> MAVASTRLPTVGCSCSVATLAYSRTYVRSSNTRSTGSSSGSIISSSLPWSQHRCQVRTLIVPRQLKAYGGTFSQSIGE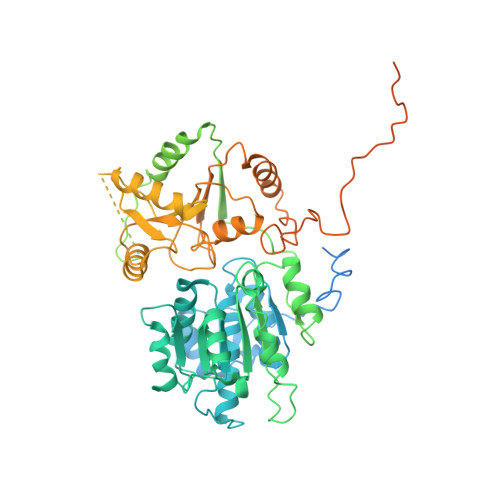RVDHAASHQVLQSLSPARTAQSPLLAKPVKTKVVDNFADMLVTPALQEALADMGVSTPSPIQQTAIEAVLQRKNTVIAAPHGEGKTLAYLLPLYQNMEKDRDVYKIPLRERRPRMILLAPTKELVEQLQTVCARLDAATGLTSVCFTSRKRSKYHLSRMLKNTMADVLVMDPKLILRLLRTRRLFIEDLRYFAVDEADAMMSSLHDHDAVQLLMKVQKRNQFKYLWPVQTQYVFVTAYMTRKLEYIVGRKISDPVTCMFRQLMHRPQARLRHRFYAIRREPEKFTVLMHLLRKNGHVPLPIDTDVAEVDVHTNPRKLSGSLAEWHEAVQRCAWKEQHEQEKSSGSGEAVTDDVVDVDEVAVRAPEEASAAVPSVGLSATENAAADDDYDHDSYARYTLERVRPLHWEHLTTVAAPFTCPIRRTVFAEGRRTIIFFRNIDATTAVFHQLRSAGFAVSLLHASLPYKVRKEMYADFASGRTNILCATDVAARGLDLHVDMVINFDVPTNALAYLSRSGRTARMGREGQVLNLYNKHQGVIVSAIKAFLKDNLPMEGLTNRKADMMQPRYAEWRTHKINALARSYVSLITRKTIPAHLERTYVHHNATWRPVFHPQKTGIHGGVAPRQQQKLMDRVREQAVWFRRGQLARRKGGRAKFGSRTMKHGVWNDIGGVASREVVNEAQNPSPAGPNFGPPSGPPQ>YKKAGLQRTLVLIKPDAFERSLVAEIMGRIEKKNFKIVSMKFWSKAPRNLIEQHYKEHSEQSYFNDLCDFMVSGPIISIVYEGTDAISKIRRLQGNILTPGTIRGDLANDIRENLIHASD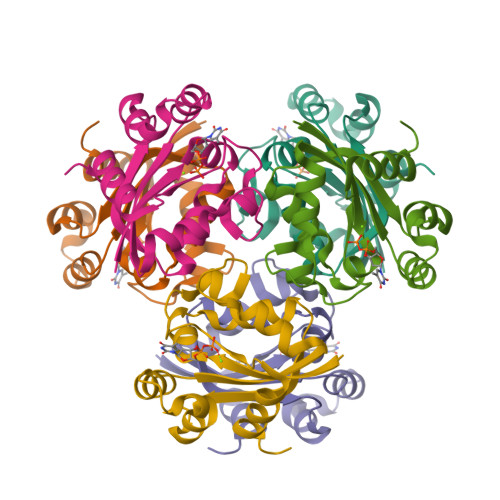SEDSAVDEISIWFPETKMETDN[6x]> GHMSTFIFPGDSFPVDPTTPVKLGPGIYCDPNTQEIRPVNTGVLHVSAKGKSGVQTAYIDYSSKRYIPSVNDFVIGVIIGTFSDSYKVSLQNFSSSVSLSYMAFPNASKKNRPTLQVGDLVYARVCTAEKELEAEIECFDSTTGRDAGFGILEDGMIIDVNLNFARQLLFNNDFPLLKVLAAHTKFEVAIGLNGKIWVKCEELSNTL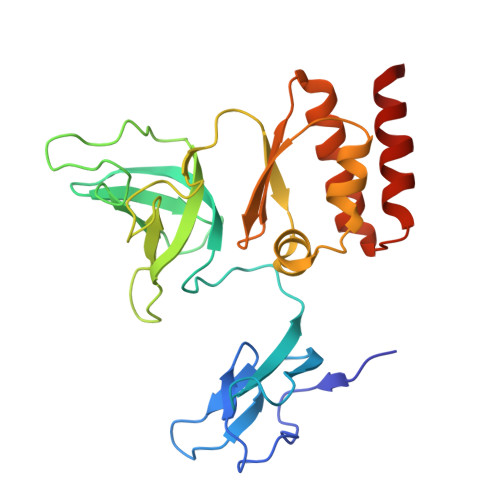ACYRTIMECCQKNDTAAFKDIAKRQFKEILTVKEE> MFEKLYSAIIYSDEFKKILLGRGVDDLEIASAYIAFLYEDLPIIGKNLCAAFLRMGLDAVYNVMPSGKVYSPRHKLYPISRYGIDGVCINCDGGKIILRISNKGYDPEDLLESKGLESRIFVSKNFKKKSMEIIEKIWDVNKIRLIARKEILERISAGGILHMIRLEHHHHHH

Genome segregation is a fundamental process that preserves the genetic integrity of all organisms, but the mechanisms driving genome segregation in archaea remain enigmatic. This study delved into the unknown function of SegC (SSO0033), a novel protein thought to be involved in chromosome segregation in archaea. The segC (sso0033) gene encodes a 165-residue hypothetical protein of unknown function. SegC has a tertiary structure folding similar to those of the ThDP-binding fold superfamily, but SegC shares only 5–15% sequence identity with those proteins. Surprisingly, we found that SSO0033 exhibits nucleotide triphosphatase (NTPase) activity and assembles into filaments in the presence of nucleoside triphosphates (NTPs) and DNA.

During the crystallization trials, we also observed another crystal form under different condition after a couple of months of crystal screening. After further structural determination, we were surprised to find that only monomer structure was present in the asymmetric unit, hereafter referred to as SegCm. The r.m.s.d. between the SegCm and SegC monomers is 0.42 Å (in Cα), implying that the overall structure does not change much. However, the electron density in the C-terminal region of SegCm (residues 155–165) is missing. The loss of the C-terminal region of SegCm (residues 155–165) may result in an inability to form the AB dimer interface, thereby disrupting dimer formation. To confirm that the missing C-terminus was not due to a flexibility issue, we dissolved SegCm crystals and measured their molecular weight by mass spectrometry. The results of mass spectrometry showed two main peaks for the SegCm crystal of 18038.6 Da and 18143.8 Da, which were significantly smaller than the molecular weight peak for SegC (19859.7 Da). This difference in molecular weight corresponds to a peptide of approximately fourteen residues (including six his-tag), implying that residues after Gly159 are degraded during crystallization. Thus, the extreme C-terminal region of SegC is crucial for dimer formation, as its degradation destroys the AB dimer interface, preventing dimer assembly and even further affecting the genesis of multimers.> MTKKVGLLVMAYGTPYKDEDIERYYTDIRHGH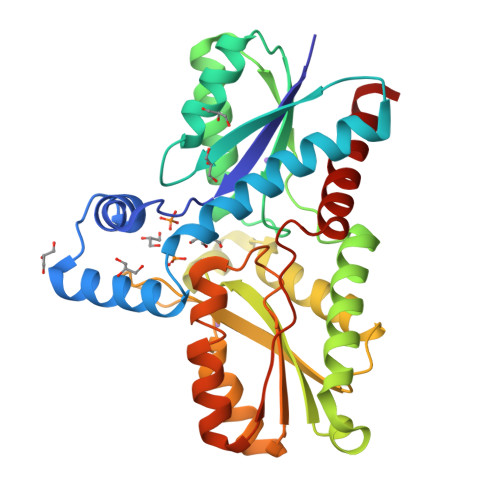KPSEEMIADLRGRYHAIGGLSPLAKITEAQAYGLEKALNDSQDEVEFKAYIGLKHIEPFIEDAVEAMHKDGIEEAISIVLAPHYSSFSVEAYNKRAKEAADKLGGPRINAINDWYKQPKFIQMWADRINETAKQIPADELLDTVLIVSAHSLPEKIKQHNDPYPNQLQETADFIFEKVVVPHYALGWQSEGKTGEPWLGPDVQDLTRELYGREKYKHFIYTPVGFVAEHLEVLYDNDYECKVVTDEVGAAYHRPPMPNSDPEFLEVLRTVVWEKYSNLEH9-(5-{[(3S)-3-amino-3-carboxypropyl][3-(3-carbamoylphenyl)propyl]amino}-5-deoxy-alpha-D-ribofuranosyl)-9H-purin-6-amine 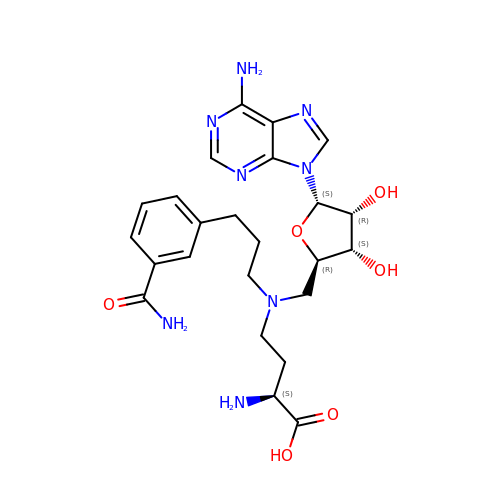| C24 H32 N8 O6 | VSETVFOQAVXGIV-LWXSJTDASA-N>[4x]MASPELRQEFQQLIQEFQQLLQEIQQLIRELLKIKLQIIKQLREASEKARNPEKKSVLQKQLELEEKQIELL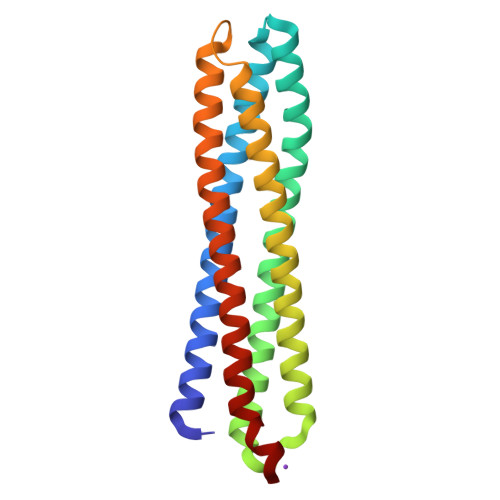ETLQQTAQEAQQLLQELQQTGQELWQLGGSGGPELRQKFQQLAQKIQQLLQKFQQLVAKQLEDEEKFIELLETILGGSGGDELRELLKGKLQVIKQQRELLQLVQKAQQLVQKLQQTGQKLWENLYFQ>[4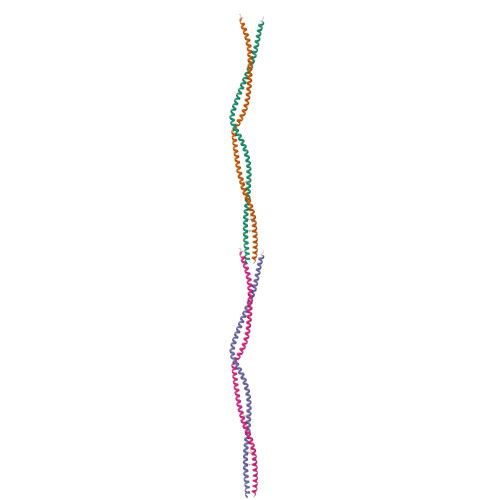x]MDKLREKINAARAETDEAVARAEAAEAKLKEVELQLSLKEQEYESLSRKSEAAESQLEELEEETKQLRLKADNEDIQKTEAEQLSRKVELLEEELETNDKLLRETTEKMRQTDVKAEHFERRVQSLERERDDMEQKLEEMTDKYTKVKAELDEVHQALEDL> AAAAAAAAAAAAAAAAAAAAAAAAAAAAAAAAAAAAAAAAAAAAAAA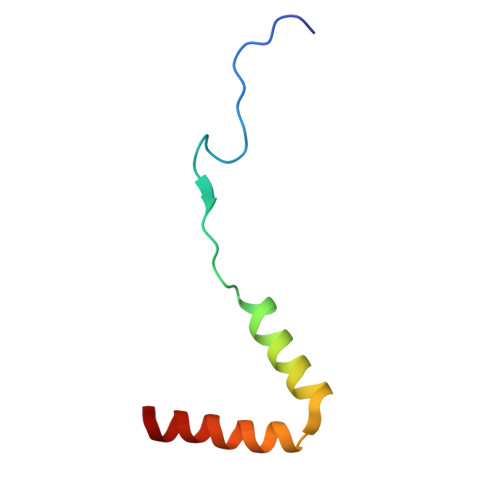AAAAAAAAA> SELLVNTKSGKVMGTRVPVLSSHISAFLGIPFAEPPVGNMRFRRPEPKKPWSGVWNASTYPNNCQQYVDEQFPGFSGSEMWNPNREMSEDCLYLNIWVPSPRPKSTTVMVWIYGGGFYSGSSTLDVYNGKYLAYTEEVVLVSLSYRVGAFGFLALHGSQEAPGNVGLLDQRMALQWVHDNIQFFGGDPKTVTIFGESAGGASVGMHILSPGSRDLFRRAILQSGSPNCPWASVSVAEGRRRAVELGRNLNCNLNSDEELIHCLREKKPQELIDVEWNVLPFDSIFRFSFVPVIDGEFFPTSLESMLNSGNFKKTQILLGVNKDEGSFFLLYG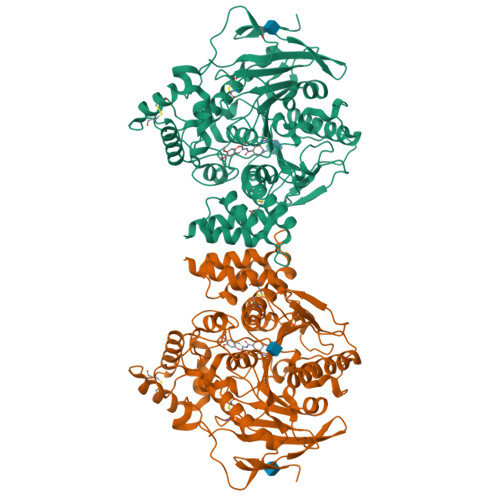APGFSKDSESKISREDFMSGVKLSVPHANDLGLDAVTLQYTDWMDDNNGIKNRDGLDDIVGDHNVICPLMHFVNKYTKFGNGTYLYFFNHRASNLVWPEWMGVIHGYEIEFVFGLPLVKELNYTAEEEALSRRIMHYWATFAKTGNPNEPHSQESKWPLFTTKEQKFIDLNTEPMKVHQRLRVQMCVFWNQFLPKLLNATETIDEAERQWKTEFHRWSSYMMHWKNQFDHYSRHESCAEL(2S)-2,3-disulfanylpropan-1-ol 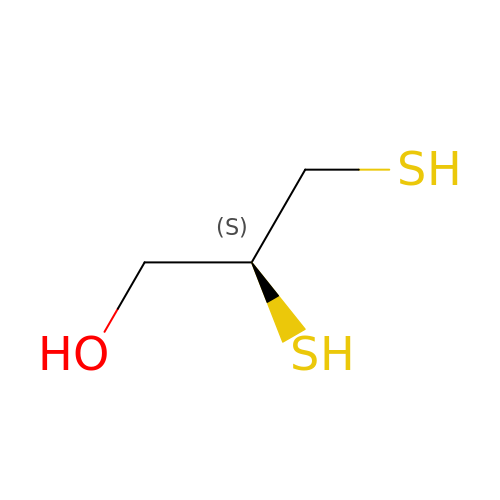| C3 H8 O S2 | WQABCVAJNWAXTE-VKHMYHEASA-N Sirtuins constitute a conserved family of nicotinamide adenine dinucleotide (NAD+)-dependent lysine deacylases with seven members known as SIRT1–7 in mammals. SIRT3, a member of the sirtuin family of NAD+-dependent protein deacylase, is critical for DLBCL growth and survival. SIRT3 deacetylates a broad variety of mitochondrial proteins involved in cellular metabolism. Among sirtuins, SIRT1, 2, and 3 share similar enzymatic activities, which is challenging for the design of SIRT3 specific inhibitors.

Among many of the inhibitors we tried, we were able to obtain the X-ray crystal structures of SIRT3 in complex with NH6-10, which has high aqueous solubility and facilitated the crystallization process. The complex appears to crystallize as a weakly associating dimer, and the unit cell parameters are unique among the human SIRT3 structures. The inhibitor resides at the interface of the two chains related by noncrystallographic symmetry and forms several favorable contacts with the opposite chain, which complicates the design somewhat. NH6-10 formed a covalent adduct with the cosubstrate NAD+ as expected. While most residues near the NH6-10 binding sites in the three sirtuins are identical, we identified two residues, P297 and E325, that can differentiate SIRT3 from SIRT1 and SIRT2. P297 of SIRT3 interacts with the benzene ring of NH6-10. In the SIRT1 and SIRT2 structures, the residues corresponding to SIRT3 P297 are N417 and S238, respectively, which cannot interact with the benzene ring of NH6-10. The second SIRT3-unique residue, E325, likely interacts with the positively charged triethylammonium at the C-terminus of NH6-10. The corresponding residues are Q267 in SIRT2 and R446 in SIRT1. To understand the improved potency, we obtained X-ray crystallography structures of human SIRT3 in a complex with an SJ-106C analog (NH6-10). This structure revealed two small molecule–protein interactions that may contribute to its better potency: the Cbz group packs against P297 of SIRT3, and the positively charged triethylammonium may interact with the negatively charged E325 of SIRT3.

>[2x]SDKGKLSLQDVAELIRARACQRVVVMVGAGISTPSGIPDFRSPGSGLYSNLQQYDLPYPEAIFELPFFFHNPKPFFTLAKELYPGNYKPNVTHYFLRLLHDKGLLLRLYTQNIDGLERVSGIPASKLVEAHGTFASATCTVCQRPFPGEDIRADVMADRVPRCPVCTGVVKPDIVFFGEPLPQRFLLHVVDFPMADLLLILGTSLEVEPFASLTEAVRSSVPRLLINRDLVGPLAWHPRSRDVAQLGDVVHGVESLVELLGWTEEMRDLVQRETGKLDGPDK>MKTIIINGVQFNTDEDTTILKFARDNNIDISALCFLNNCNNDINKCEICTVEVEGTGLVTACDTLIEDGMIINTNSDAVNEKIKSRISQLLDIHEFKCGPCNRRENCEFLKLVIKYKARASKPFLPKDKTEYVDERSKSLTVDRTKCLLCGRCVNACGKNTETYAMKFLNKNGKTIIGAEDEKCFDDTNCLLCGQCIIACPVAALSEKSHMDRVKNALNAPEKHVIVAMAPSVRASIGELFNMGFGVDVTGKIYTALRQLGFDKIFDINFGADMTIMEEATELVQRIENNGPFPMFTSCCPGWVRQAENYYPELLNNLSSAKSPQQIFGTASKTYYPSISGLDPKNVFTVTVMPCTSKKFEADRPQMEKDGLRDIDAVITTRELAKMIKDAKIPFAKL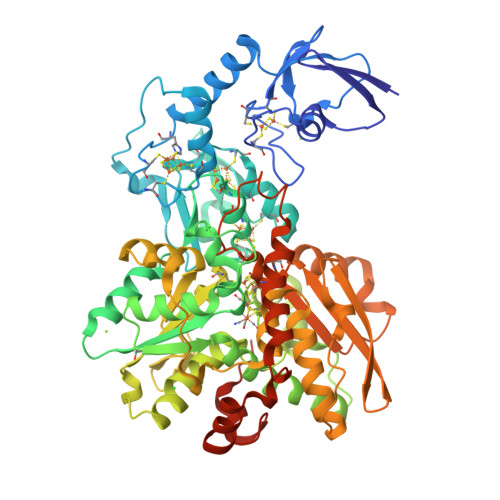EDSEADPAMGEYSGAGAIFGATGGVMEAALRSAKDFAENAELEDIEYKQVRGLNGIKEAEVEINNNKYNVAVINGASNLFKFMKSGMINEKQYHFIEVMACHGGCVNGGGQPHVNPKDLEKVDIKKVRASVLYNQDEHLSKRKSHENTALVKMYQNYFGKPGEGRAHEILHFKYKKSAWSHPQFEK[2x]[(2~{E},6~{E},10~{E},14~{E},18~{Z},22~{E},26~{Z},30~{E},34~{E},38~{E})-3,7,11,15,19,23,27,31,35,39,43-undecamethyltetratetraconta-2,6,10,14,18,22,26,30,34,38,42-undecaenyl] 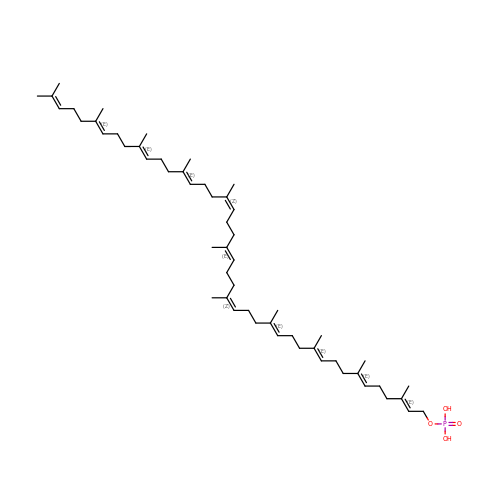dihydrogen phosphate | C55 H91 O4 P | UFPHFKCTOZIAFY-ZUPWODLNSA-N>EVYGIIAMQAAYRDYDSGDAKQDDNLGGMQLNNESRIGFRGKKQFANFEP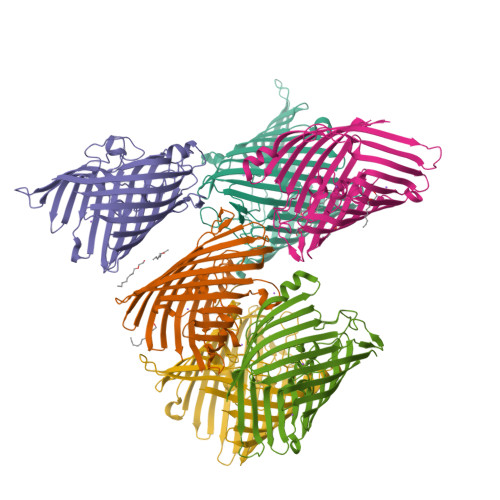TFIWQIEGGYVDPSFGGEGAGLGERDTFVGFESASWGQVRLGRVLTPMYELVDWPASNPGLGDVYDWGGAIGGAKYQDRQSNTIRWDSPMYADKFSIDAAVGAGDKAGLGAGDDYWGGIAAHYKLGPLQLDAAYEGNRNIEAEGQTWENNTYLVGVQGWFENGISFFAQYKYMEADASNGVNEKQDAMSAGLMYTTGDWQYKLGYAANFDLERDGKTLSNTSDDVVSAQIMYFVDPSAVLYARARMNDFNEGLDGLDDAARWTSGTNGDYNEYSVGVEYYF[6x];> DGANSD(3S,4S,7Z)-7-(2-amino-1,3-thiazol-4-yl)-4-formyl-1-[({3-(5-hydroxy-4-oxo-3,4-dihydropyridin-2-yl)-4-[3-(methylsulfonyl)propyl]-5-oxo-4,5-dihydro-1H-1,2,4-triazol-1-yl}sulfonyl)amino]-3,10,10-trimethyl-1,6-dioxo-9-oxa-2,5,8-triazaundec-7-en-11-oic 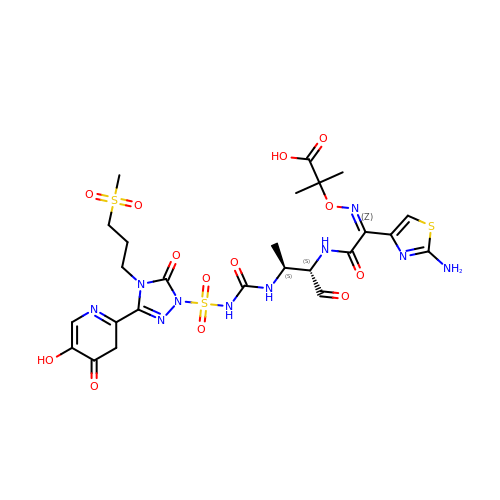acid | C25 H32 N10 O13 S3 | KOZNTWBICKFGGR-BECCELLYSA-N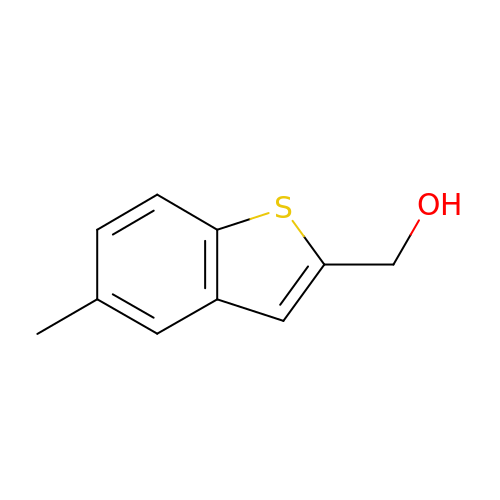(5-methyl-1-benzothiophen-2-yl)methanol | C10 H10 O S | NPSSZIBANMLQHP-UHFFFAOYSA-N>MDHRTSIAQAMVDRISKQMDGSQPDEYFNNLYGNVSRQTYKFEEIREFPYVAVHIGTETGQYLPSGQQWMFLELPILVYDKEKTDIQEQLEKLVADIKTVIDTGGNLEYTVSKPNGSTFPCEATDMIITSVSTDEGLLAPYGLAEINVTVRYQPPRRSLRR[6x];>MSLQLLRNTRIFVSTVKTGHNKTNTQEILVQDDISWGQDSNSTDITVNEAGPRPTRGSKRFNDSLNAAEWSFSTYILPYKDKNTSKQIVPDYMLWHALSSGRAINLEGTTGAHNNATNFMVNFKDNSYHELAMLHIYILTDKTWSYIDSCQINQAEVNVDIEDIGRVTWSGNGNQLIPLDEQPFDPDQIGIDDETYMTIQGSYIKNKLTILKIKDMDTNKSYDIPITGGTFTINNNITYLTPNVMSRVTIPIGSFTGAFELTGSLTAYLNDKSLGSMELYKDLIKTLKVVNRFEIALVLGGEYDDERPAAILVAKQAHVNIPTIETDDVLGTSVEFKAIPSDLDAGDEGYLGFSSKYTRTTINNLIVNGDGATDAVTAITVKSAGNVTTLNRSATLQMSVEVTPSSARNKEVTWAITAGDAATINATGLL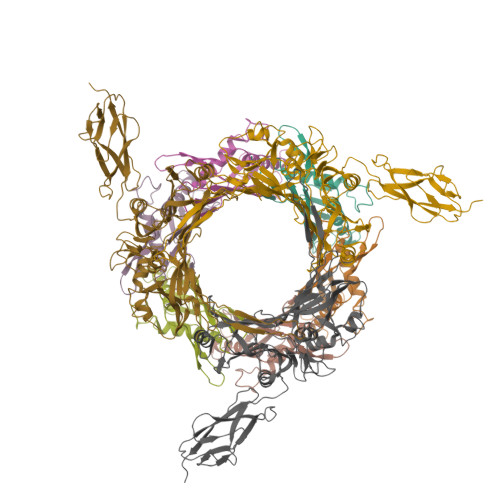RADASKTGAVTVEATAKDGSGVKGTKVITVTAGG[3x]> MGIIRTCRLGPDQVKSMRAALDLFGREFGGVATYSQHQPDSDYLGNLLRSKTFIALAAFDQEAVVGALAAYVLPKFEQARSEIYIYDLAVSGEHRRQGIATALINLLKHEANALGAYVIYVQADYGDDPAVALYTKLGIREEVMHFDIDPSTAT

The primary mode of resistance to aminoglycoside antibiotics is through chemical modification catalyzed by aminoglycoside-modifying enzymes. Here we present the first structural and functional studies of two aminoglycoside-modifying enzymes that do not use target mimicry, AAC(3)-Ia and AAC(3)-XIa. X-ray diffraction studies reveal that these enzymes bind aminoglycoside antibiotics in a conformation where the central 2-deoxystreptamine ring is in boat conformation. Similar to other AACs, AAC(3)-Ia and AAC(3)-XIa display the GNAT superfamily fold.

We have determined two crystal structures of AAC(3)-Ia from Acinetobacter baumannii and five of AAC(3)-XIa from C. striatum, in complex with various aminoglycosides and either CoASH or AcCoA, as well as a structure where one of two active sites contains AcCoA. Both AAC(3)-Ia structures only contain a single protomer per asymmetric unit. In the AAC(3)-Ia structure, sisomicin is present in both antibiotic binding sites of the dimer. The experimental maps of the antibiotics in all AAC(3)-Ia and AAC(3)-XIa ternary complex structures presented in this report unambiguously place the aminoglycosides’ central ring in a boat conformation rather than the canonical chair conformation. Additionally, in all of these aminoglycosides the N-3, O-4 and O-5 atoms of the central ring were positioned in an axial plane rather than an equatorial plane, positioning the prime ring of aminoglycoside around 90° to the central ring. In the AAC(3)-Ia and AAC(3)-XIa complexes, regions of the adjacent protomer in the swapped dimer contribute to the aminoglycoside binding sites. In both structures, the C-terminal swapped dimer tail from the adjacent protomer makes direct contact with the aminoglycoside. A glutamic acid residue forms a hydrogen bond with N-3” in AAC(3)-Ia and N-3” in and N-1 in AAC(3)-XIa. In AAC(3)-Ia, the aminoglycoside site is opened and easy for ligands to access, whereas in AAC(3)-XIa, the aminoglycoside binding site is closed off and the enzyme would require a conformational shift to accept reactants and release products. Whereas AAC(3)-IIIa only made contacts with the central ring and the double prime ring, leaving the prime ring solvent exposed. In total, the boat-binder AAC(3)-Ia made 16 hydrogen bonds with sisomicin, and AAC(3)-XIa made 17 hydrogen bonds with acetylated sisomicin, while AAC(3)-IIIa only made 7 hydrogen bonds with sisomicin.> SEAEARPTNFIRQIIDEDLASGKHTTVHTRFPPEPNGYLHIGHAKSICLNFGIAQDYKGQCNLRFDDTNPVKEDIEYVESIKNDVEWLGFHWSGNVRYSSDYFDQLHAYAIELINKGLAYVDELTPEQIREYRGTLTQPGKN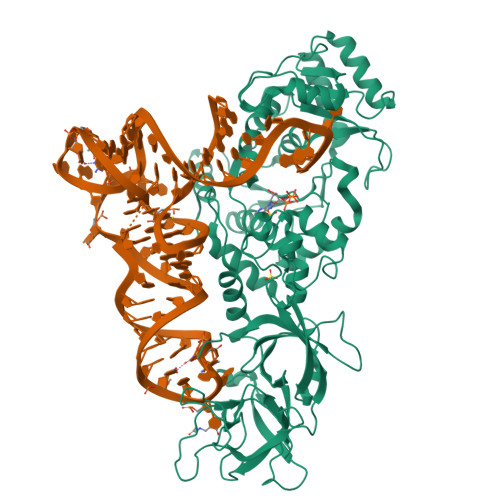SPYRDRSVEENLALFEKMRAGGFEEGKACLRAKIDMASPFIVMRDPVLYRIKFAEHHQTGNKWCIYPMYDFTHCISDALEGITHSLCTLEFQDNRRLYDWVLDNITIPVHPRQYEFSRLNLEYTVMSKRKLNLLVTDKHVEGWDDPRMPTISGLRRRGYTAASIREFCKRIGVTKQDNTIEMASLESCIREDLNENAPRAMAVIDPVKLVIENYQGEGEMVTMPNHPNKPEMGSRQVPFSGEIWIDRADFREEANKQYKRLVLGKEVRLRNAYVIKAERVEKDAEGNITTIFCTYDADTLSKDPADGRKVKGVIHWVSAAHALPVEIRLYDRLFSVPNPGAADDFLSVINPESLVIKQGFAEPSLKDAVAGKAFQFEREGYFCLDSRHSTAEKPVFNRTVGLRDTWAKVGE>[3x]MKSIHIKIVLALCISIFTIMGLQPLNQHSTVAAANHKSSTKQTPLTFVLIHGSWATAGFWDETASELRKLGHTVYTPEYAGHGADKNNNVTHEQITKSVVDYI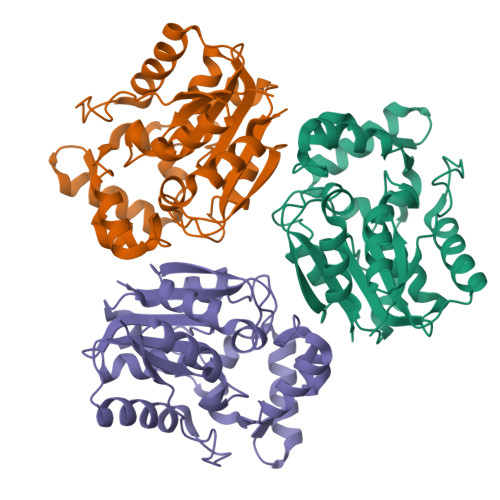KQKDLKDFILLGHSFGGSVIQTVSQQVPDRIKRIVFFDAFAPLDGQSVADQFPAESLKSFEQLRDASGNNTITLPFPLFRDTFVNTASLAQAQAFYKQAPPEPATPLFEKLDLKKFYSLQIPKSYLYLTEDTAIPQGPYGFHPTQSSHLGVFRFIEGKGDHMTTVRTEPKMMAELMVKAGRD Staufen proteins bind structured mRNA motifs through dsRNA-binding domains (dsRBD) and are involved in mRNA localization in Drosophila and mammals. Members of the Stau protein family share a common domain organization, consisting of four to five copies of the dsRNA-binding domain (dsRBD) separated by linkers that are predicted to be unstructured. Similarly, a stem of 19 bp is required for the binding of human Stau1 (hStau1) to the 3ʹUTR of ADP-Ribosylation Factor 1 (ARF1) mRNA. To understand how Stau recognizes its target RNAs, we determined the crystal structure of the minimal RNA-binding region of hStau1, consisting of dsRBDs 3 and 4, in complex with the 19 bp SBS from ARF1 mRNA.

To test if binding of hStau1 induces conformational changes in the target RNA, we determined the structure of the ARF1 SBS in isolation, at 1.9 Å resolution. The crystals belong to space group H32, with the asymmetric unit (ASU) including one and half RNA molecules, co-axially stacked. This arrangement generates a sixfold static disorder, as previously observed in crystal structures of dsRNAs of similar length. The refined ARF1 SBS model has an Rfree of 24.8% and Rfactor of 22.6%, with good stereochemistry. The ARF1 SBS forms a blunt end duplex with standard A-form helix conformation and Watson–Crick base pairing throughout, except for two wobble base pairs. A comparison with the structure of unbound ARF1 SBS, at 1.9 Å resolution, reveals that the target RNA undergoes minor changes upon hStau1 binding. We do not observe major conformational changes in ARF1 SBS upon hStau1 binding. The structural models of apo and bound ARF1 SBS superpose well, with 1.32 Å root mean square deviation. Overall, bound ARF1 SBS is slightly more stretched than in its unbound state, resulting in a slight widening of the major groove at points engaged in interaction with the helix α2 of dsRBD3A and dsRBD3B. Moreover, small displacements of ∼4 Å take place at both 3′ and 5′ end of the ARF1 sense strand, in regions contacted by the β1–β2 loop of dsRBD3A and dsRBD3B.

> GAGUGCCAGAAGCUGCCUC;> GAGUGCCAGA;> GAGGCAGUUUCUGGUACUC;> CUGGUACUC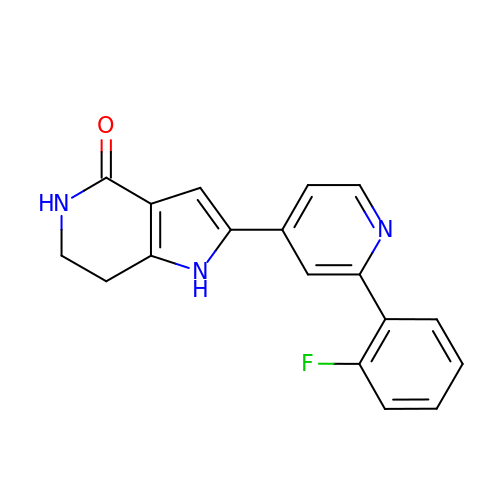2-[2-(2-FLUOROPHENYL)PYRIDIN-4-YL]-1,5,6,7-TETRAHYDRO-4H-PYRROLO[3,2-C]PYRIDIN-4-ONE | C18 H14 F N3 O | XJJYJNMNYDNXNO-UHFFFAOYSA-N>IKTLSVSRPIIYGNTAKKMGSVKPPNAPAEHTHLWTIFVRGPQNEDISYFIKKVVFKLHDTYPNPVRSIEAPPFELTETGWGEFDINIKVYFVEEANEKVLNFYHRLRLHPYANPVPNSDNGNEQNTTDHNSKDAEVSSVYFDEIVFNEPNEEFFKILMS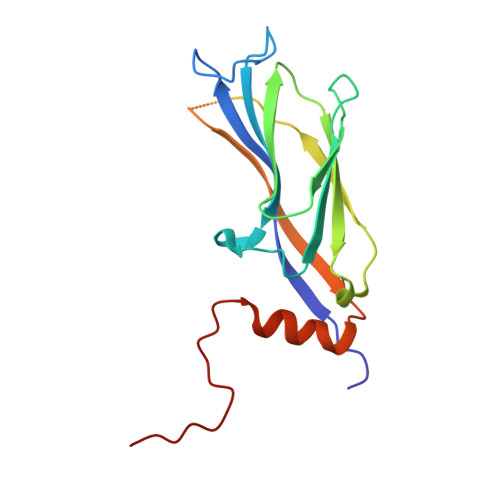RPGNLLPSLERPHRD[2x]> ASTT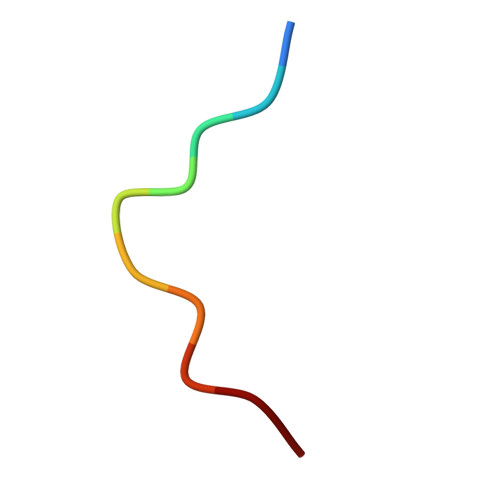GANSQR>MKIVKDFSPKEYSQKLVNWLSDSCMNYPAEGFVIGLSGGIDSAVAASLAVKTGLPTTALILPSDNNQHQDMQDALELIEMLNIEHYTISIQPAYEAFLASTQSFTNLQNNRQLVIKGNAQARLRMMYLYAYAQQYNRIVIGTDNACEWYMGYFTKFGDGAADILPLVNLKKSQVFELGKYLDVP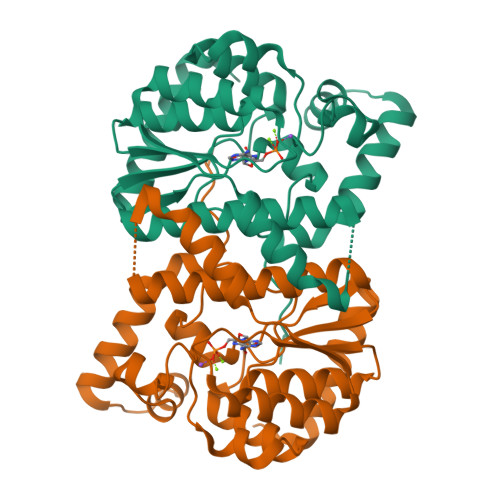KNILDKAPSAGLWQGQTDEDEMGVTYQEIDDFLDGKQVSAKALERINFWHNRSHHKRKLALTPNF[4x]> KIEDIGQGAEIIKRTQDITSKRLAITQNIQFDFVKDKKYNKDALVVKMQGFISSRTTYSDLKKYPYIKRMIWPFQYNISLKTKDSNVDLINYLPKNKIDSADVSQKLGYNIGSFNYSKTISYNQKNYVTEVESQNSKGVKWGVKANSFVTPNGQVSAYDQYLFAQDPTGPAARDYFVPDNQLPPLIQSGFNPSFITTLSHERGK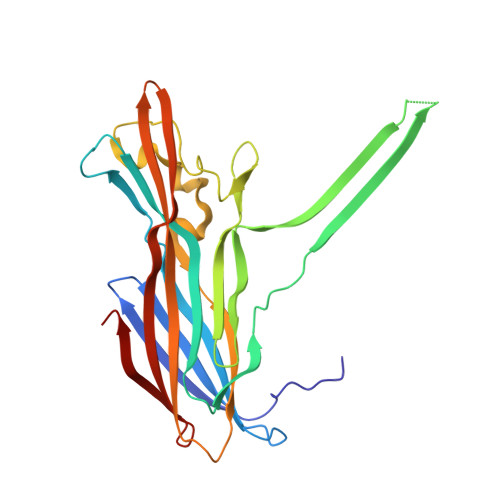GDKSEFEITYGRNMDATYAYVTRHRLAVDRKHDAFKNRNVTVKYEVNWKTHEVKIKSITPK> YRAFDIYNDKVAGFAKFLKTNCCRFQEKDEDDNLIDSYFVVKRHTFSNYQHEETIYNLLKDCPAVAKHDFFKFRIDGDMVPHISRQRLTKYTMADLVYALRHFDEGNCDTLKEILVTYNCCDDDYFNKKDWYDFVENPDILRVYANLGERVRQALLKTVQFCDAMRNAGIVGVLTLDNQDLNGNWYDFGDFIQTTPGSGVPVVDSYYSLLMPILTLTRALTAESHVDTDLTKPYIKWDLLKYDFTEERLKLFDRYFKYWDQTYHPNCVNCLDDRCILHCANFNVLFSTVFPPTSFGPLVRKIFVDGVPFVVSTGYHFRELGVVHNQDVNLHSSRLSFKELLVYAADPAMHAASGNLLLDKRTTCFSVAALTNNVAFQTVKPGNFNKDFYDFAVSKGFFKEGSSVELKHFFFAQDGNAAISDYDYYRYNLPTMCDIRQLLFVVEVVDKYFDCYDGGCINANQVIVNNLDKSAGFPFNKWGKARLYYDSMSYEDQDALFAYTKRNVIPTITQMNLKYAISAKNRARTVAGVSICSTMTNRQFHQKLLKSIAATRGATVVIGTSKFYGGWHNMLKTVYSDVENPHLMGWDYPKCDRAMPNMLRIMASLVLARKHTTCCSLSHRFYRLANECAQVLSEMVMCGGSLYVKPGGTSSGDATTAYANSVFNICQAVTANVNALLSTDGNKIADKYVRNLQHRLYECLYRNRDVDTDFVNEFYAYLRKHFSMMILSDDAVVCFNSTYASQGLVASIKNFKSVLYYQNNVFMSEAKCWTETDLTKGPHEFCSQHTMLVKQGDDYVYLPYPDPSRILGAGCFVDDIVKTDGTLMIERFVSLAIDAYPLTKHPNQEYADVFHLYLQYIRKLHDELTGHMLDMYSVMLTNDNTSRYWEPEFYEAMYTPHT;> DKRAKVTSAMQTMLFTMLRKLDNDALNNIINNARDGCVPLNIIPLTTAAKLMVVIPDYNTYKNTCDGTTFTYASALWEIQQVVDADSKIVQLSEISMDNSPNLAWPLIVTALRA;> KMS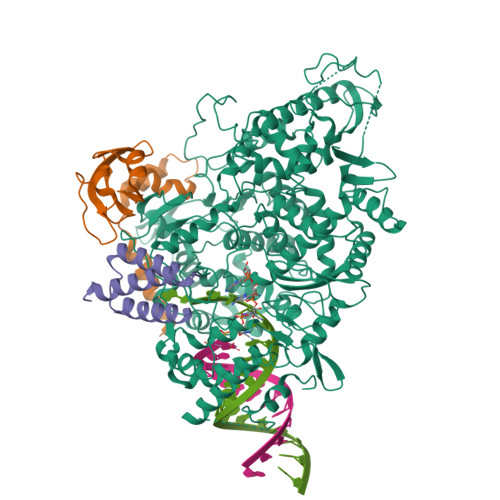DVKCTSVVLLSVLQQLRVESSSKLWAQCVQLHNDILLAKDTTEAFEKMVSLLSVLLSMQG> MDKINLVCGSLLHNIGKIIYRGTSERAKHSKLGGDFIKSFEQFRNTELTDCIRYHHAQEITSVKSN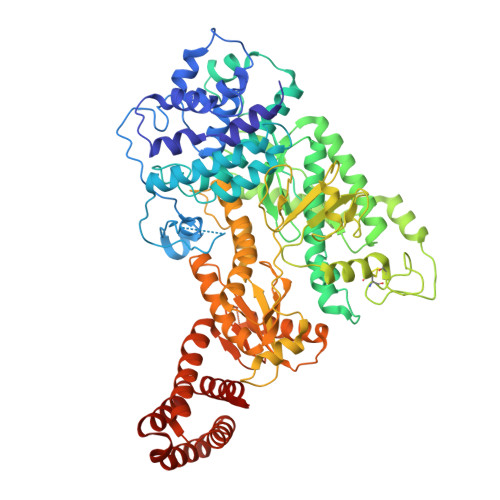KEKNSLFYITYIADNISSGMDRRKDLEEGAEGFNWDKKVALGSVFNVLNEKEKGRQNYSYPFVARTRIKEEPLNFPTATQNQYTTSYYDGLITDMKTILQRLKPDKEHINSLLQMMESLWSYVPSSTDKNQLVDISLYDHSRTTAAIASAIYDYFQAENITDYQKELFDYNATEFYDKNAFLMMNFDMSGVQNFIYNISGSKALKSLRARSFYLDMLLEYISDNLLEKLELSRANILYVGGGHAYLLLANTNKTKAILSDFEHDLKTWFLDKFKIDLYVAMAYTEVSANDLMNHNGHYRDIYRRLSQKTSAKKANRYTAEEILNLNHQGTENARECRECKRSDLLIEEDDICEICDSLQKVSRDLTRENIFVIANEGVLDMPFGKKMSALSYSQADKLKKSNAEVQIYAKNISEIGQNLMTRIDMGDYTYRSDFHEMLEEVEVGINRLGVLRADVDNLGQAFINGIPDDYLSISRTATFSRAMSRFFKNYLNQLLAEKSYKINVIYAGGDDLFMIGAWQDILDFSIVLKQKFADFTQNKLSISAGIGMFREKYPVARMASLTGDLEDAAKDYKPDERAVQATKNAVTLFDATNVFSWDTLENDIFVKLDAITKNFEKLDETGKAFIYRLIDLLRGVNENQQINIARLAYTLSRMEEKIGKTFAQELYNWANADRKTLIMALEIYILKTRE>[2x]MLNQELELSLNMAFARAREHRHEFMTVEHLL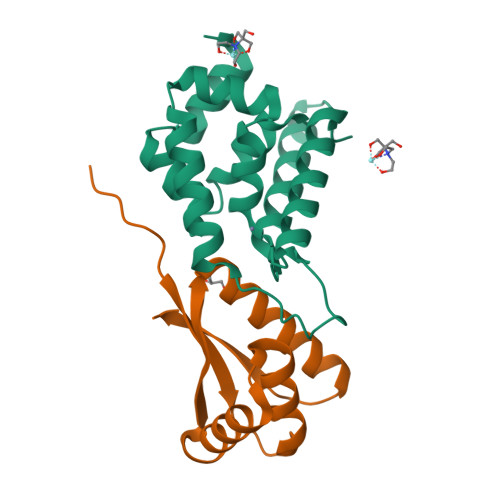LALLSNPSAREALEACSVDLVALRQELEAFIEQTTPVLPASEEERDTQPTLSFQRVLQRAVFHVQSSGRNEVTGANVLVAIFSEQESQAAYLLRKHEVSRLDVVNFISHGT;>[2x]MGKTNDWLDFDQLAEEKVRDALKPPSMYKVILVNDDYTPMEFVIDVLQKFFSYDVERATQLMLAVHYQGKAICGVFTAEVAETKVAMVNKYARENEHPLLCTLEKA>[4x]MTGLAEAIANTVQAAQQHDSVK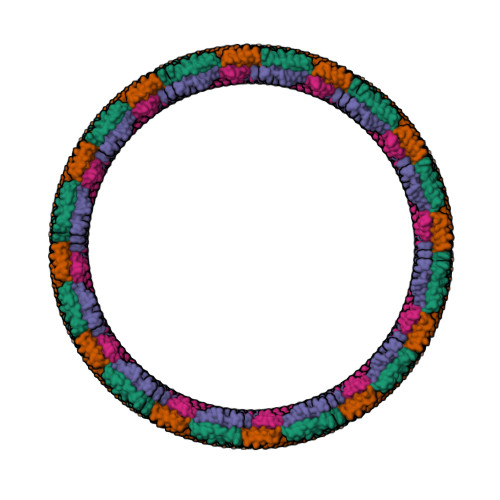LGTSIVDIVANGVGLLGKLFGF> GLVPRGSHMTAQTVTGAVAAAQLGATLPHEHVIFGYPGYAGDVTLGPFDHAAALASCTETARALLARGIQTVVDATPNDCGRNPAFLREVSEATGLQILCATGFYYEGEGATTYFKFRASLGDAESEIYEMMRTEVTEGIAGTGIRAGVIKLASSRDAITPYEQLFFRAAARVQRETGVPIITHTQEGQQGPQQAELLTSLGADPARIMIGHMDGNTDPAYHRETLRHGVSIAFDAIGLQGMVGTPTDAERLSVLTTLLGEGYADRLLLSHDSIWHWLGRPPAIPE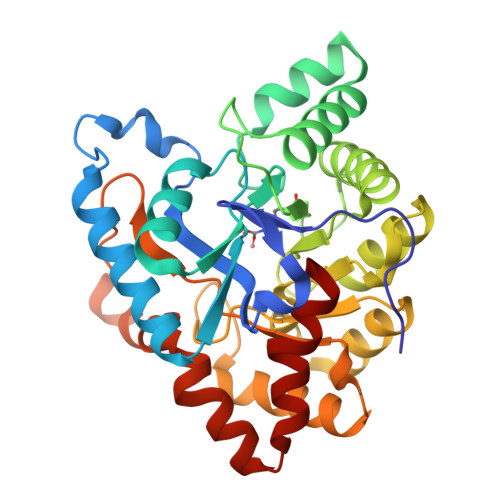AALPAVKDWHPLHISDDILPDLRRRGITEEQVGQMTVGNPARLFG> GAMVLDPEVAQLLSQANEAFVRNDLQVAERLFNEVIKKDARNFAAYETLGDIYQLQGRLNDCCNSWFLAAHLNASDWEFWKIVAILSADLDHVRQAIYCFSRVISLNPMEWESIYRRSMLYKKTGQLARALDGFQRLYMYNPYDANILRELAILYVDYDRIEDSIELYMKVFNANVERREAILAALENALDSSDEESAAEGEDADEKEPLEQDEDRQMFPDINWKKIDAKYKCIPFDWSSLNILAELFLKLAVSEVDGIKTIKKCARWIQRRESQTFWDHVPDDSEFDNRRFKNSTFDSLLAAEKEKSYNIPIDIRVRLGLLRLNTDNLVEALN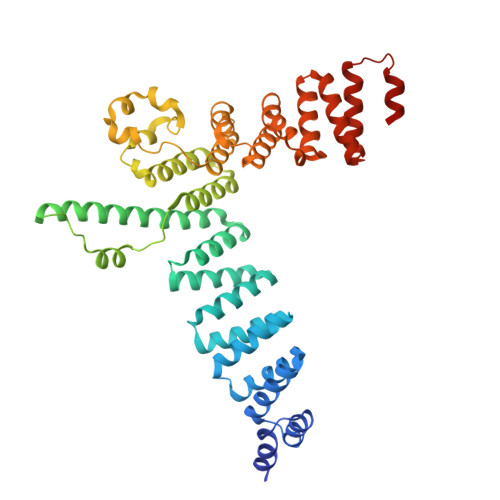HFQCLYDETFSDVADLYFEAATALTRAEKYKEAIDFFTPLLSLEEWRTTDVFKPLARCYKEIESYETAKEFYELAIKSEPDDLDIRVSLAEVYYRLNDPETFKHMLVDVVEMR>GGHHWTYEGPHGQDHWPTSYPECGGDAQSPINIQTDSVIFDPDLPAVQPHGYDQLGTEPLDLHNNGHTVQLSLPPTLHLGGLPRKYTAAQLHLHWGQRGSLEGSEHHINSEATAAELHVVHYDSQSYSSLSEAAQKPQGLAVLGILIEVGETENPAYDHILSRLHEIRYKDQKTSVPPFSVRELFPQQLEQFFRYNGSLTTPPCYQ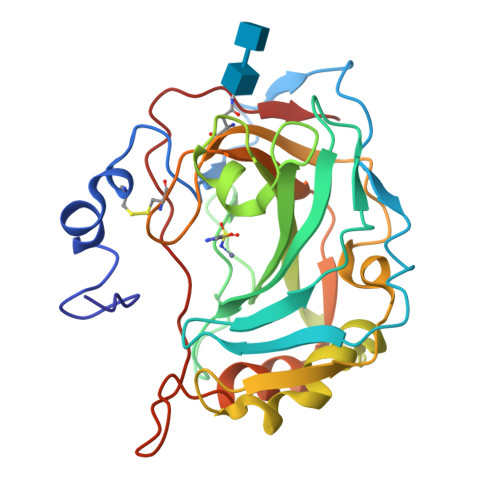SVLWTVFNRRAQISMGQLEKLQETLSSTEEDPSEPLVQNYRVPQPLNQRTIFASF[2x]> QYAPQTQSGRTSIVHLFEWRWVDIALECERYLGPKGFGGVQVSPPNENIVVTNPSRPWWERYQPVSYKLCTRSGNENEFRDMVTRCNNVGVRIYVDAVINHMCGSGAAAGTGTTCGSYCNPGNREFPAVPYSAWDFNDGKCKTASGGIESYNDPYQVRDCQLVGLLDLALEKDYVRSMIADYLNKLIDIGVAGFRIDASKHMWPGDIKAVLDKLHNLNTNWFPAGSRPFIFQEVIDLGGEAIQSSEYFGNGRVTEFKYGAKLGTVVRKWSGEKMSYLKNWGE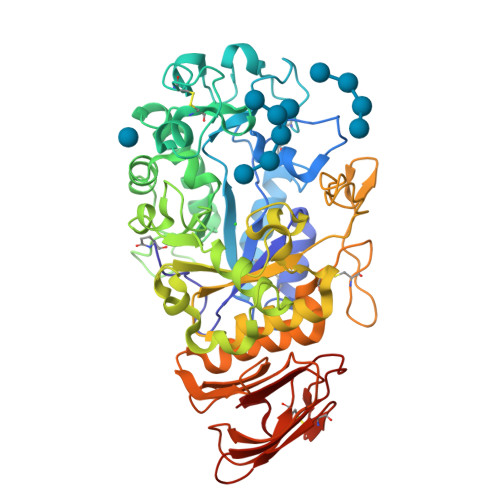GWGFMPSDRALVFVDNHDNQRGHGAGGASILTFWDARLYKVAVGFMLAHPYGFTRVMSSYRWARNFVNGQDVNDWIGPPNNNGVIKEVTINADTTCGNDWVCEHRWRQIRNMVWFRNVVDGQPFANWWDNGSNQVAFGRGNRGFIVFNNDDWQLSSTLQTGLPGGTYCDVISGDKVGNSCTGIKVYVSSDGTAQFSISNSAEDPFIAIHAESKL> GPGGSMITVNEKEHILEQKYRPSTIDECILPAFDKETFKSITSKGKIPHIILHSPSPGTGKTTVAKALCHDVNADMMFVNGSDCKIDFVRGPLTNFASAASFDGRQKVIVIDEFDRSGLAESQRHLRSFMEAYSSNCSIIITANNIDGIIKPLQSRCRVITFGQPTDEDKIEMMKQMIRRLTEICKHEGIAIADMKVVAALVKKNFPDFRKTIGELDSYSSKGVLDAGILSLVTNDRGAIDDVLESLKNKDVKQLRALAPKYAADYSWFVGKLAEEIYSRVT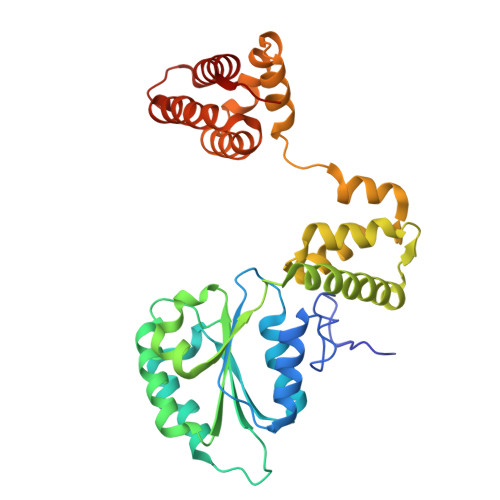PQSIIRMYEIVGENNQYHGIAANTELHLAYLFIQLACEMQWK> GHMLIPHDLLEADTLNNLLEDFVTREGTDNGDETPLDVRVERARHALRRGEAVILFDPESQ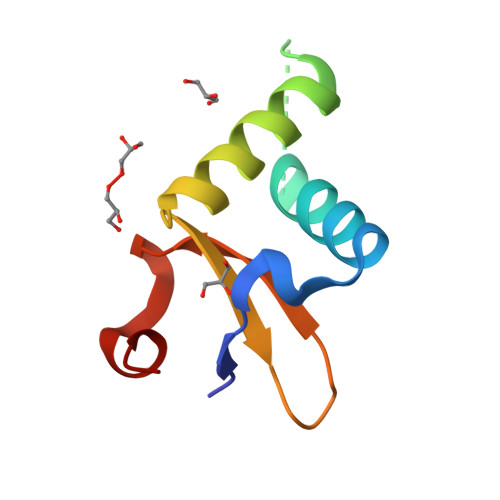QCQLMLRSEVPAELLRD>MGSRDHLFKVLVVGDAAVGKTSLVQRYSQDSFSKHYKSTVGVDFALKVLQWSDYEIVRLQLWDIAGLERFAAMTRLYYRDASACVIMFDVTNATTFSNSQRWKQDLDSKLTLPNGEPVPCLLLANKCDLSPWAVSRDQIDRFSKENGFTGWTETSVKENKNINEAMRVLIEKMMRNS[2x];>[2x]MASGSCQGCEEDEETLKKLIVRLNNVQEGKQIETLVQILEDLLVFTYSEHASKLFQGKNIHVPLLIVLDSYMRVASVQQVGWSLLCKLIEVCPGTMQSLMGPQDVGNDWEVLGVHQLILKMLTVHNASVNLSVIGLKTLDLLLTSGKITLLILDEESDIFMLIFDAMHSFPANDEVQKLGCKALHVLFERVSEEQLTEFVENKDYMILLSALTNFKDEEEIVLHVLHCLHSLAIPCNNVEVLMSGNVRCYNIVVEAMKAFPMSERIQEVSCCLLHRLTLGNFFNILVLNEVHEFVVKAVQQYPENAALQISALSCLALLTETIFLNQDLEEKNENQENDDEGEEDKLFWLEACYKALTWHRKNKHVQEAACWALNNLLMYQNSLHEKIGDEDGHFPAHREVMLSMLMHSSSKEVFQASANALSTLLEQNVNFRKILLSKGIHLNVLELMQKHIHSPEVAESGCKMLNHLFEGSNTSLDIMAAVVPKILTVMKRHETSLPVQLEALRAILHFIVPGMPEESREDTEFHHKLNMVKKQCFKNDIHKLVLAALNRFIGNPGIQKCGLKVISSIVHFPDALEMLSLEGAMDSVLHTLQMYPDDQEIQCLGLSLIGYLITKKNVFIGTGHLLAKILVSSLYRFKDVAEIQTKGFQTILAILKLSASFSKLLVHHSFDLVIFHQMSSNIMEQKDQQFLNLCCKCFAKVAMDDYLKNVMLERACDQNNSIMVECLLLLGADANQAKEGSSLICQVCEKESSPKLVELLLNSGSREQDVRKALTISIGKGDSQIISLLLRRLALDVANNSICLGGFCIGKVEPSWLGPLFPDKTSNLRKQTNIASTLARMVIRYQMKSAVEEGTASGSDGNFSEDVLSKFDEWTFIPDSSMDSVFAQSDDLDSEGSEGSFLVKKKSNSISVGEFYRDAVLQRCSPNLQRHSNSLGPIFDHEDLLKRKRKILSSDDSLRSSKLQSHMRHSDSISSLASEREYITSLDLSANELRDIDALSQKCCISVHLEHLEKLELHQNALTSFPQQLCETLKSLTHLDLHSNKFTSFPSYLLKMSCIANLDVSRNDIGPSVVLDPTVKCPTLKQFNLSYNQLSFVPENLTDVVEKLEQLILEGNKISGICSPLRLKELKILNLSKNHISSLSENFLEACPKVESFSARMNFLAAMPFLPPSMTILKLSQNKFSCIPEAILNLPHLRSLDMSSNDIQYLPGPAHWKSLNLRELLFSHNQISILDLSEKAYLWSRVEKLHLSHNKLKEIPPEIGCLENLTSLDVSYNLELRSFPNEMGKLSKIWDLPLDELHLNFDFKHIGCKAKDIIRFLQQRLKKAVPYNRMKLMIVGNTGSGKTTLLQQLMKTKKSDLGMQSATVGIDVKDWPIQIRDKRKRDLVLNVWDFAGREEFYSTHPHFMTQRALYLAVYDLSKGQAEVDAMKPWLFNIKARASSSPVILVGTHLDVSDEKQRKACMSKITKELLNKRGFPAIRDYHFVNATEESDALAKLRKTIINESLNFKIRDQLVVGQLIPDCYVELEKIILSERKNVPIEFPVIDRKRLLQLVRENQLQLDENELPHAVHFLNESGVLLHFQDPALQLSDLYFVEPKWLCKIMAQILTVKVEGCPKHPKGIISRRDVEKFLSKKRKFPKNYMTQYFKLLEKFQIALPIGEEYLLVPSSLSDHRPVIELPHCENSEIIIRLYEMPYFPMGFWSRLINRLLEISPYMLSGRERALRPNRMYWRQGIYLNWSPEAYCLVGSEVLDNHPESFLKITVPSCRKGCILLGQVVDHIDSLMEEWFPGLLEIDICGEGETLLKKWALYSFNDGEEHQKILLDDLMKKAEEGDLLVNPDQPRLTIPISQIAPDLILADLPRNIMLNNDELEFEQAPEFLLGDGSFGSVYRAAYEGEEVAVKIFNKHTSLRLLRQELVVLCHLHHPSLISLLAAGIRPRMLVMELASKGSLDRLLQQDKASLTRTLQHRIALHVADGLRYLHSAMIIYRDLKPHNVLLFTLYPNAAIIAKIADYGIAQYCCRMGIKTSEGTPGFRAPEVARGNVIYNQQADVYSFGLLLYDILTTGGRIVEGLKFPNEFDELEIQGKLPDPVKEYGCAPWPMVEKLIKQCLKENPQERPTSAQVFDILNSAELVCLTRRILLPKNVIVECMVATHHNSRNASIWLGCGHTDRGQLSFLDLNTEGYTSEEVADSRILCLALVHLPVEKESWIVSGTQSGTLLVINTEDGKKRHTLEKMTDSVTCLYCNSFSKQSKQKNFLLVGTADGKLAIFEDKTVKLKGAAPLKILNIGNVSTPLMCLSESTNSTERNVMWGGCGTKIFSFSNDFTIQKLIETRTSQLFSYAAFSDSNIITVVVDTALYIAKQNSPVVEVWDKKTEKLCGLIDCVHFLREVTVKENKESKHKMSYSGRVKTLCLQKNTALWIGTGGGHILLLDLSTRRLIRVIYNFCNSVRVMMTAQLGSLKNVMLVLGYNRKNTEGTQKQKEIQSCLTVWDINLPHEVQNLEKHIEVRKELAEKMRRTSVE

Mutations in the LRRK2 gene, which encodes the leucine-rich repeat kinase 2 (LRRK2) protein, are among the most frequent genetic causes of late-onset PD and account for ~5% of familial and ~1% of sporadic cases. Most LRRK2-related PD mutations, such as G2019S (Gly2019→Ser), have increased kinase activity. Previous studies have suggested an emerging “Rab29–LRRK2–Rabs” cascade for LRRK2 signaling, in which GTP-bound Rab29 (Rab29•GTP) facilitates LRRK2 membrane recruitment and activation, then activated LRRK2 phosphorylates Rab GTPases, including Rab29 itself.

We determined cryo–electron microscopy (cryo-EM) structures of the Rab29–LRRK2 complex, reconstituted by mixing LRRK2, Rab29EM, GTP analog (GppNHp), adenosine triphosphate (ATP), and Mg2+. We thus introduced three point mutations (Q67L, T71A, and S72A) to Rab29 (Rab29EM) to maximize the opportunity of capturing the active Rab29•GTP–LRRK2 complex (where Q is glutamine, L is leucine, T is threonine, A is alanine, and S is serine). T71A and S72A prevent Rab29 phosphorylation, and Q67L abolishes GTPase activity and enhances the interaction between Rab29 and LRRK2 (26). The observation of LRRK2 dimers both in the presence and absence of Rab29 suggests that COR-B–mediated dimerization of LRRK2 could occur under physiological settings.>[2x]HHHHHHHHGSSLEVLFQGPAVASADGDAPSPVSVSASAATKGPSSSSVLTFQQAIQRLQDYWASVGCAVMQCSNTEVGAGTMNPLTFLRVLGPEPWNVAYVEPSIRPDDSRYGDNPNRLQRHTQFQVILKPDPGNSQDLFLHSLSALGINVREHDIRFVEDNWESPVLGAWGLGWEVWMDGMEITQFTYFQQSGSLPLLPVSVEITYGLERILMSLQGVDHFKNIQYTKGITYGELFLENEKEMSAYYLEHANVDNIQKHFDDFEEEARSLLSLWLPIPAYDHVLKASHAFNILDSRGFVGVTERARYFGRMRSLARQCAQLWVKTRENLGYPLGTYQESNLIYPHVSEKPSRKGVVGQPRAFVLEIGTEELPPHDVIEATKQLEKSLIQILEKRRLSHGKVRSYGTPRRLAVVVENLNMKQMEEEIELRGPPVAKAFDQEGRPTKAAEGFCRKNNVPIDSLYRRTDGKTEYIYARVKESARFADEVLTEDLPTIISGISFPKSMRWNSNIVFSRPIRWIFALHGDLIVPFCFAGISSGNQSCGLRNSSLANFKVEAAELYLHTLEKAGILIDMQERKQRILHDSSILAEGVGGDIIAPDSLVQEVINLVEAPMPIIGRYDVSFLALPKDVLITVMQKHQKYFPVTSKTMGNLLPCFITVANGAIKEEVVRKGNEAVLRARYEDAKFFYKMDTQKKLSEFRDQLSSILFHERLGTMLDKMKRVENTVAEVALLLGINEKMIPAIKDAAALAMSDLATNIVTEFTSLAGIMARHYALRDGLSEQIAEALFEITLPRFSGDVFPKTDPGIVLAVTDRLDSLVGLFGAGCQPSSTNDPFGLRRISYGLVQILVENKKNFDLTKALTLVAEEQPITIDSGVIDEVVQFVTRRLEQLLVDEGINCEIVRSVLIERANCPYLASQTAIEMEAFSRTEDFPKIVEAYSRPTRIIRGKEIGSALEVDASVFEKDEERALW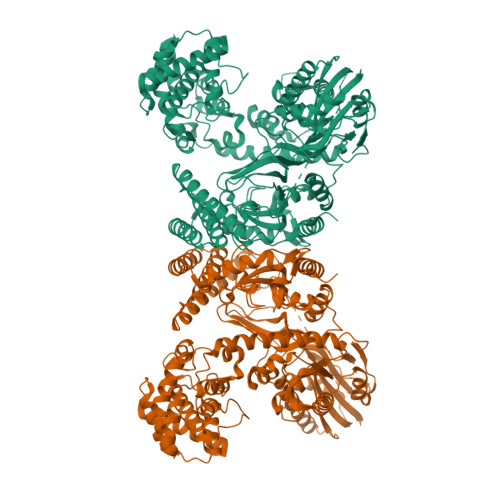SAYLEVADKIHPGVDIKAFADASLELLQPLEDFFTNVFVMAEDEKVRNNRLALLTKVASLPKGIADLSVLPGF> GSMPKPINVRVTTMDAELEFAIQPNTTGKQLFDQVVKTVGLREVWFFGLQYVDSKGYSTWLKLNKKVTQQDVKKENPLQFKFRAKFFPEDVSEELIQEITQRLFFLQVKEAILNDEIYCPPETAVLLASYAVQAKYGDYNKEIHKPGYLANDRLLPQRVLEQHKLTKEQWEERIQNWHEEHRGMLREDSMMEYLKIAQDLEMYGVNYFEIKNKKGTELWLGVDALGLNIYEHDDKLTPKIGFPWSEIRNISFNDKKFVIKPI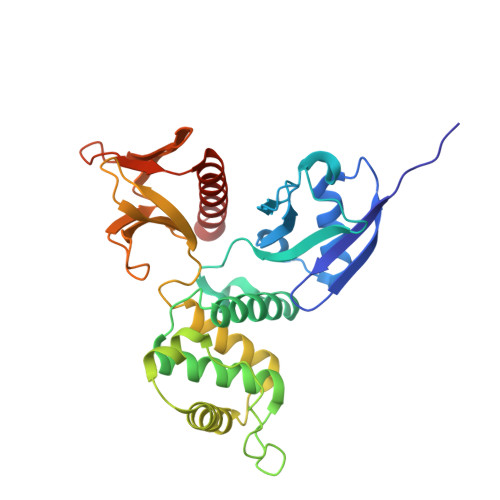DKKAPDFVFYAPRLRINKRILALCMGNHELYMRRRK>MIESLADWSIFTDPDVFGEPVTWTTPPLPDPVPAIFTDASEDRPATLGPGVLTIAPTLTLGAAQLPFSPARNHRCTVRGITYRVAEVQPDGSGGLRLLLERV[6x];>[6x]MLKGKDGVVKNASTGDSIGHLQSWALDTQRDEVSGWGMGDDAERAFTTVGRASGNFEVYLDPADPSDDLEPGDLVDLELYPGGESTGSGYRSVAGALILSTAESASKDGIPMLTVNWRTSGALPQKATVS;>MSEAIIAAARGRLISPPFSDATGDVYRTPEAALPAIIVELDYTDAERISMGGGFIASAELRVEI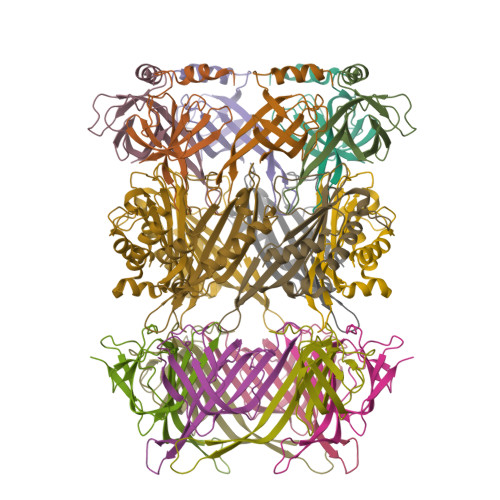LAKRDDWSLLTPTPANTAEGMARLAALVRTAILAPPSDLSGLAWSIAPAGYEFETERGETPLARATQSFALQILQP[6x]> KK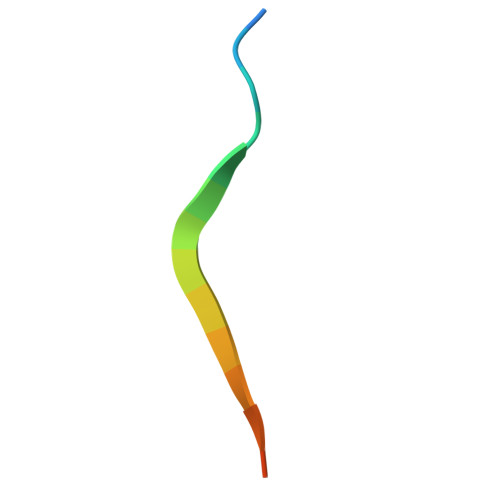GSVVIVGRIILSGRK~{N}2-methyl-~{N}4-[(1~{R},5~{S})-3-oxabicyclo[3.1.0]hexan-6-yl]-6-[(1~{S})-1-phenylethyl]pyridine-2,4-dicarboxamide 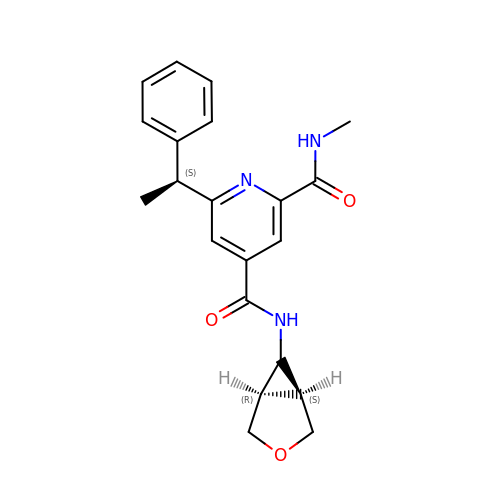| C21 H23 N3 O3 | VTIIKJCRYRUFLT-NALNUFGESA-N> APTSSSTKKTQLQLEHLLLDLQMILNGINNYKNPKLTRMLTFKFYMPKKATELKHLQCLEEELKPLEEVLNLAQSKNFHLRPRDLISNINVIVLELKGSETTFMCEYADETATIVEFLNRWITFCQSIISTLT;> AVQGTSQFTCFYNSRAQISC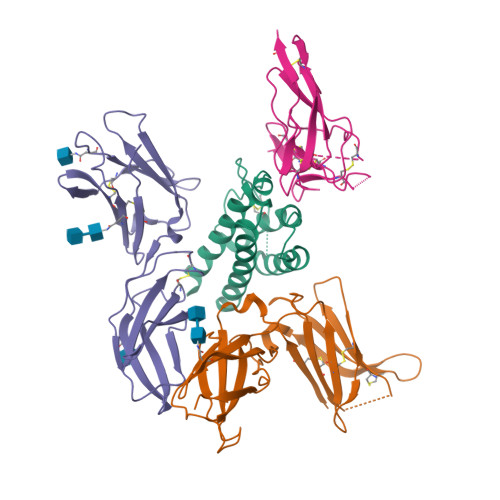VWSQDGALQDTSCQVHAWPDRRRWQQTCELLPVSQASWACNLILGAPDSQKLTTVDIVTLRVLCREGVRWRVMAIQDFKPFENLRLMAPISLQVVHVETHRCNISWEISQASHYFERHLEFEARTLSPGHTWEEAPLLTLKQKQEWICLETLTPDTQYEFQVRVKPLQGEFTTWSPWSQPLAFRTKPAALGKDT;> PLPEVQCFVFNVEYMNCTWQSSSEPQPTNLTLHYWYKNSDNDKVQKCSHYLFSEEITSGCQLQKKEIHLYQTFVVQLQDPREPRRQATQMLKLQNLVIPWAPENLTLHKLSESQLELNWNNRFLNHCLEHLVQYRTDWDHSWTEQSVDYRHKFSLPSVDGQKRYTFRVRSRFNPLCGSAQHWSEWSHPIHWGSNTSKEN;> ELCDDDPPEIPHATFKAMAYKEGTMLNCECKRGFRRIKSGSLYMLCTGNSSHSSWDNQCQCTSSATRQTTKQVTPQPEEQKERKTTEMQSPMQPVDQASLPGHCREPPPWENEATERIYHFVVGQMVYYQCVQGYRALHRGPAESVCKMTHGKTRWTQPQLICTGEMETSQFPGEEKPQASPEGRPESETSCLVTTTDFQIQTEMAATMETSIFTTE>MPAITIWGRRNSSNVRKALWCAEEAGVAYTSIEVGGAFGGNDTPAYRALNPNGVVPTLQDGALVLWESNAIVRYLAAQYAPALYPQAPAERALGDRWMDWTTSTFAGVFRDLFWGVVRTPEAERDHARIAAALTQSGELLARADAA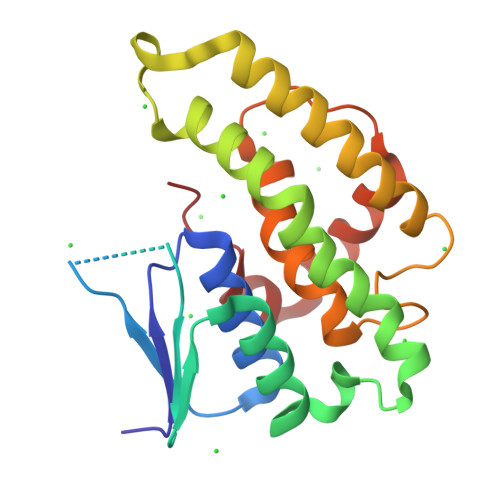LAQQPYLSGGRFAMGDIPLGSFIYAWFEMPIERPELPHLQAWYARLRVRPAYQRGVMTALT[4x]> MENTENSVDSKSIKNLEPKIIHGSESMDSGISLDNSYKMDYPEMGLCIIINNKNFHKSTGATSRSGTDVDAANLRETFRNLKYEVRNKNDLTREEIVELMRDVSKEDHSKRSSFVC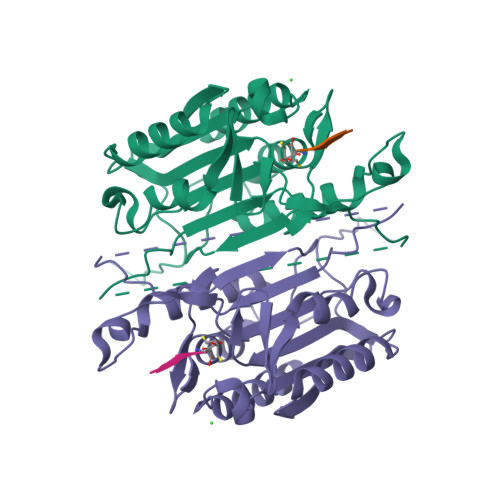VLLSHGEEGIIFGTNGPVDLKKITNFFRGDRCRSLTGKPKLFIIQACRGTELDCGIETDSGVDDDMACHKIPVEADFLYAYSTAPGYYSWRNSKDGSWFIQSLCAMLKQYADKLEFMHILTRVNRKVATEFESFSFDATFHAKKQIPCIHSMLTKELYFYHH N-[6-(5-methylsulfonylpyridin-3-yl)-[1,2,4]triazolo[1,5-a]pyridin-2-yl]ethanamide 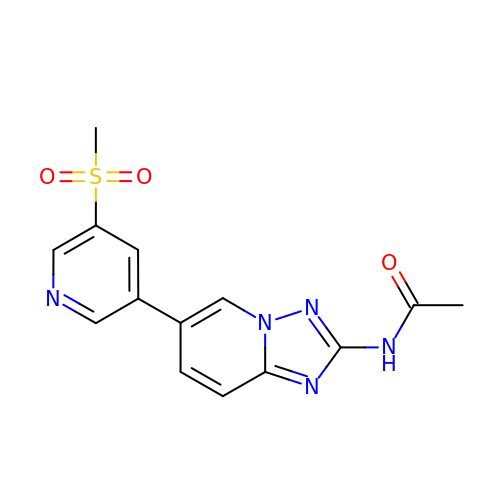| C14 H13 N5 O3 S | RCRCKEODQLBHAY-UHFFFAOYSA-N> SKYVDRVIAEVEKKYADEPEFVQTVEEVLSSLGPVVDAHPEYEEVALLERMVIPERVIEFRVPWEDDNGKVHVNTGYRVQFNGAIGPYKGGLRFAPSVNLSIMKFLGFEQAFKDSLTTLPMGGAKGGSDFDPNGKSDREVMRFCQAFMTELYRHIGPDIDVPAGDLGVGAREIGYMYGQYRKIVGGFYNGV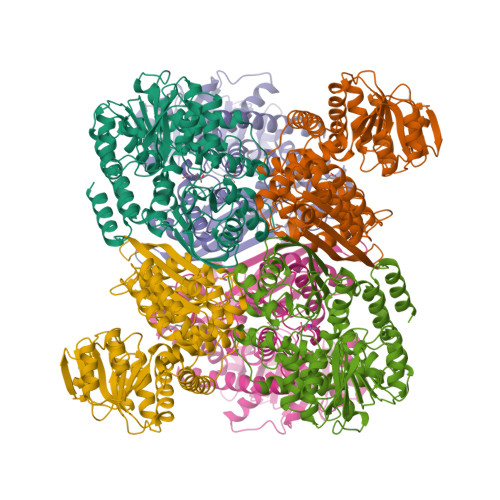LTGKARSFGGSLVRPEATGYGSVYYVEAVMKHENDTLVGKTVALAGFGNVAWGAAKKLAELGAKAVTLSGPDGYIYDPEGITTEEKINYMLEMRASGRNKVQDYADKFGVQFFPGEKPWGQKVDIIMPCATQNDVDLEQAKKIVANNVKYYIEVANMPTTNEALRFLMQQPNMVVAPSKAVNAGGVLVSGFEMSQNSERLSWTAEEVDSKLHQVMTDIHDGSAAAAERYGLGYNLVAGANIVGFQKIADAMMAQGIAW> SVKNETVKLSVGTVSGNPGDTVKVPVTISQVSTPVGLICMDISYDASKFTVKDVLPNTDL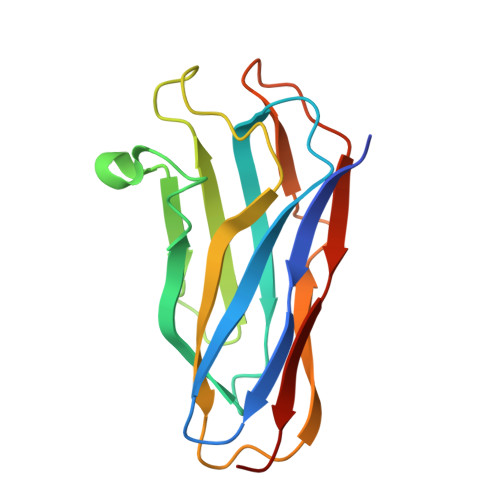VKDTDNYSFIVNTSTPGKISITFTDPTLANYPISVDGILAYLDFIINSNATAGDSALTVDPATLIVADENDKDIKDAASNGKITVTGSAP>[15x]MTTKVIFTFHNPDGSPQANEKFTVRLTRPGMSDAEHCVVIPETYEMVTDAKGEFTMDLESSTSAYRVTAIGDDDEYEDDPCSQYTFTFYV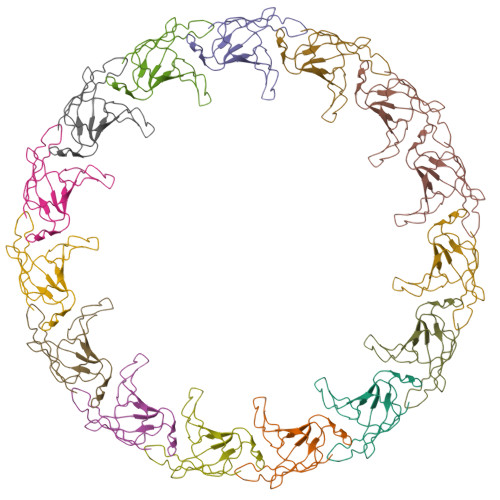PDSADPVYVQELILMPPPTNLPWDEEAMNKITQAVVDAREARDEAEAQADRAEVQVDLAKAEVVKAQDEVVKAKAEVTKAQAEVTKAAQQVELAKVEVGKAEASAAAAKVSETNAANAAAGSAASATAATNQANRAKTEADRSKSEADRARDLADAMAEKVEGGSLPPLVGMNETFTYEGTDPYRWTVSGPATAVSDGSVMRLTKTDGSGSRAFVRQAVSFPDSHWIVYMRVKTQTGTAAQNRSAQIRFIAADKKDCVVYFNINANGLVEPNTIHMQGTEGGTRNAATMFTGLSTETWLDLAVKYDAVNRHIELFRRLDTGVWQKGGGRLMVDAIKPAFIEVSSMPVAPQNWWLDLDFISVCKPNLICYGDSIAAGQNEYGVTRGSNSYNNNRNWAGTWFGKVPLYATNRNNLVLVQGVEGRRTWQYLSQLSEISNSGVKVVFMHASTNDVNDASMTMEKRTSDTQAIIDQLHAVGAQVVLFNSMQGTKAYNDASSTTVKLRDYTDQWWNTELPKVNGLAQTLDIARLIAKDGYMDPALGASDGLHLTNASAQKIADKLGQFFSNSSDTNGFASLDSPAFTGIPTVPTQTPFLPFGKTIANTEYVVTFIQDWTQRYGYGDLTMYSRTGAQLSGGGVRSGYYHVPAGAGNPLPSGLNTSLAFVDHKSYDTNKGWQLWNPAYTGRLFIRTTNSAGTWQTPVELATFTWLDDNNVTKPRTLKFMELPLFNPPGSPSLSGFVPIQDSADGGWRNLSATPTGVALLSASSAGGALSYLGGMPIANHTLPSNSIDNAALNGFYSVPSGTAGLPLGMDTTNGHAGITSVFDNVTKYQLLFPRTGGAGSYATSVFYRARSNNGWESWVRLLASNQLEGSVTTEPLTTAIFQNNGNNNQNVGRSVRFADGTQIVYATIRLTYSAVDVLQYTYTYPMGFVAPPTITVQPILGARADINDMPYFAVTSPFTYNVGNGNALVQIYRVAGYTAHSFASTSFINCAVVAVGRWK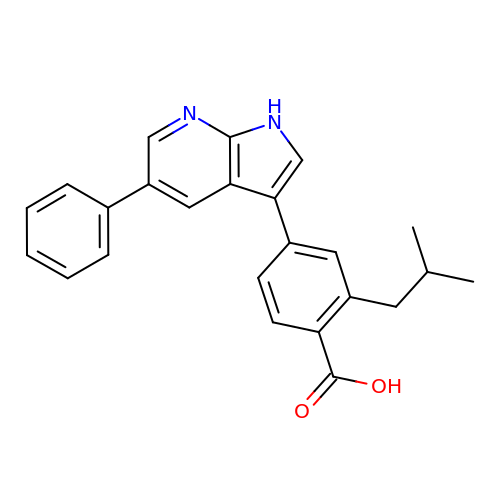2-(2-methylpropyl)-4-(5-phenyl-1H-pyrrolo[2,3-b]pyridin-3-yl)benzoic acid | C24 H22 N2 O2 | PGBYHFSGSTUFFN-UHFFFAOYSA-N> MANVIKTVLTYQLDGSNRDFNIPFEYLARKFVVVTLIGVDRKVLTINTDYRFATRTTISLTKAWGPADGYTTIELRRVTSTTDRLVDFTDGSILRAYDLNVAQIQTMHVAEEARDLTTDTIGVNNDGHLDARGRRIVNLANAVDDRDAVPFGQLKTMNQNSWQARNEALQFRNEAETFRNQAEGFKNESSTNATNTKQWRDETKGFRDEAKRFKNTAGQYATSAGNSASAAHQSEVNAENSATASANSAHLAEQQADRAEREADKLENYNGLAGAIDKVDGTNVYWKGNIHANGRLYMTTNGFDCGQYQQFFGGVTN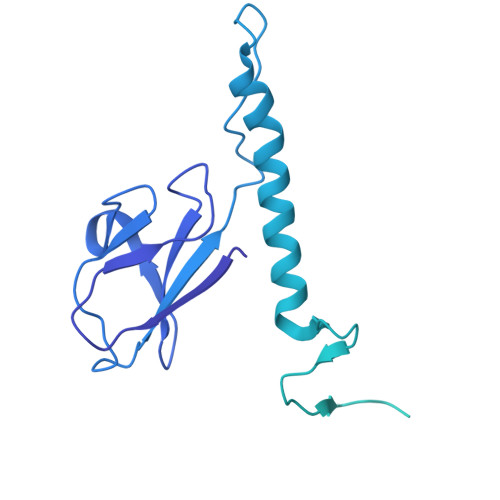RYSVMEWGDENGWLMYVQRREWTTAIGGNIQLVVNGQIITQGGAMTGQLKLQNGHVLQLESASDKAHYILSKDGNRNNWYIGRGSDNNNDCTFHSYVHGTTLTLKQDYAVVNKHFHVGQAVVATDGNIQGTKWGGKWLDAYLRDSFVAKSKAWTQVWSGSAGGGVSVTVSQDLRFRNIWIKCANNSWNFFRTGPDGIYFIASDGGWLRFQIHSNGLGFKNIADSRSVPNAIMVENE4-[4-(1-methylpiperidin-4-yl)butyl]-~{N}-(6-pyrrolidin-1-ylquinolin-5-yl)benzenesulfonamide 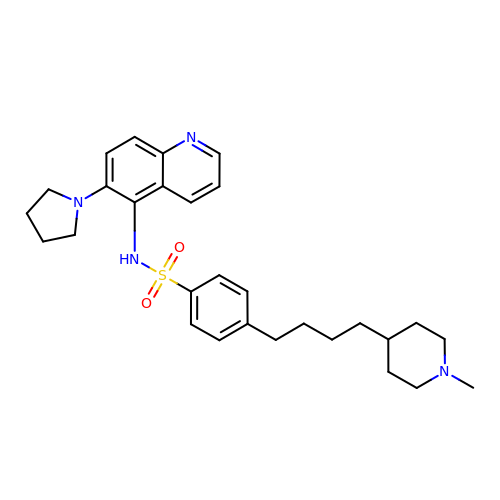| C29 H38 N4 O2 S | HRSWREJECUVHPS-UHFFFAOYSA-N>[4x]GAMAIEFDIQESKILKGVYIITPNKFRDLRGEIWTAFTDEYLSKLVPDGIKFKHDKFINSHFNVLRGIHGDVKTYKLVTCVYGEVHQVVVDCRKDSPTYL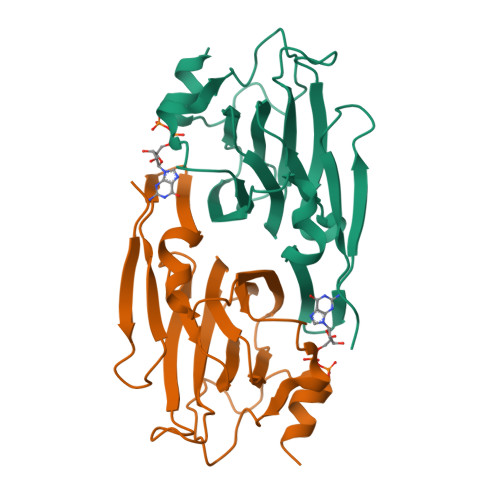KWEKFIISYKNQQLILLPPNMGNSHYVSSKEAVYYYKLAYEGEYMDAPDQFTYAWNDERIGIDWPTNTPILSDRDILATKNK>[4x]MAHHHHHHMTASDLLKPYDGLRVLVTGGASGIGLAIADAFAECGARVHVCDASQAAIAALADRPSRAAIGATLADVSDRAAVERVFADVAATLGGLDVLVNNAGIAGPTGGIDEIDPAQWEQTVAINLNAQFEFARRAVPLLRESKHGGAIIALSSVAGRLGYAYRTPYAATKWAVVGLVKSLAIELGP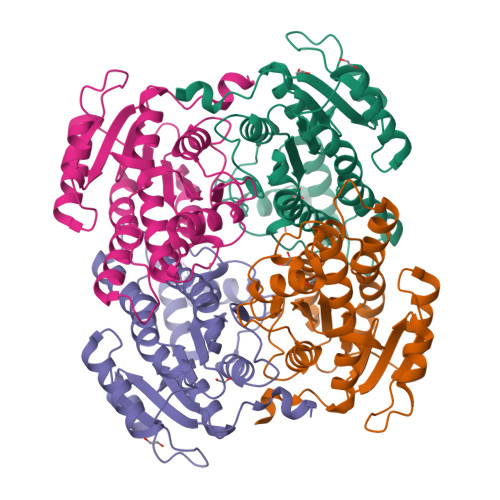LGIRVNAIQPGIVRGPRIRRVIEARAQQLGIGYDEMEQRYLERISLRRMTEPAEIAATALFLCSPGGHGITGQAISVCGNVEVL> KNTANLSLITKLSQEDGAILFPEIDRYSDNKQIKALTQQITKVTVNGTVYKDLISDSVKDTNGWVSNMTGLHLGTKAFKDGENTIVISSKGFEDVTITVTKKDGQIHFVSAKQKQH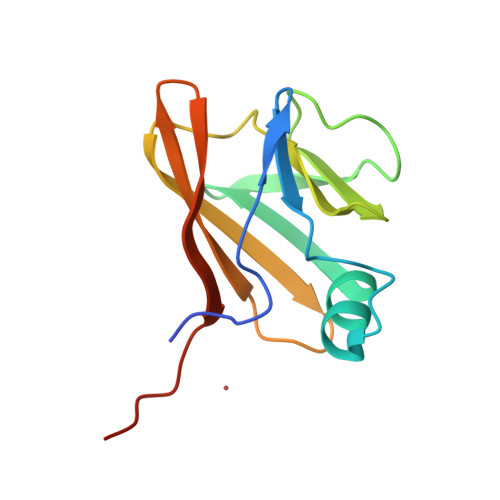VTAEDRQS4-HYDROXYBENZAMIDE | C7 H7 N O2 | 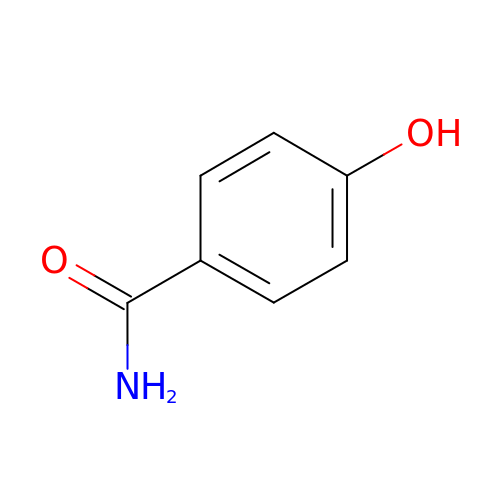QXSAKPUBHTZHKW-UHFFFAOYSA-N>[2x]SMSNRLIFDADWLVPEQVQVAGQAIQYYAARNIQYVQHPVAAIQVLNVFVPAAYLHGSSVNGYQRATAPILMPNTVGGYLPGPADDPQRVTWPTNAGTIQQALKRGYVVVAAGIRGRTTVDKSGQRVGQAPAFIVDMKAAIRYVKYNQGRLPGDANRIITNGTSAGGATSALAGASGNSAYFEPALTALGAAPATDDIFAVSAYCPIHNLEHADMAYEWQFNGINDWHRYQPVAGTTKNGRPKFEP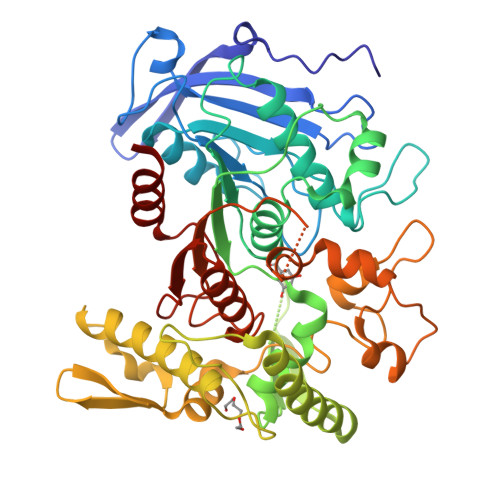VSGQLTVEEQALSLALKAQFSTYLNQLKLTASDGTHLTLNEAGMGSFRDVVRQLLISSAQTAFDQGTDIHKYAGFVVTGNQVTDLDLSAYLKSLTRMKAVPAFDQLDLTSPENNLFGDATAKAKHFTALAQTRSTVTAQLADAELIQAINPLSYLTTTSSQVAKHWRIRHGAADRDTSFAIPIILAIMLENHGYGIDFALPWDIPHSGDYDLGDLFSWIDGLCQ> KKLNLKDKYQYLTRDMAWEPTYQDKKDIFPEEDFEGIKITDWSQWEDPFRLTMDAYWKYQAEKEKKLYAIFDAFAQNNGHQNISDARYVNALKLFISGISPLEHAAFQGYSKVGRQFSGAGARVACQMQAIDELRHSQTQQHAMSHYNKHFNGLHDGPHMHDRVWYLSVPKSFFDDARSAGPFEFLTAISFSFEYVLTNLLFVPFMSGAAYNGDMATVTFGFSAQSDEARHMTLGLEVIKFILEQHEDNVPIVQRWIDKWFWRGFRLLSLVSMMMDYMLPNKVMSWSEAWEVYYEQNGGALFKDLERYGIRPPKYQDVANDAKHHLSHQLWTTFYQYCQATNFHTW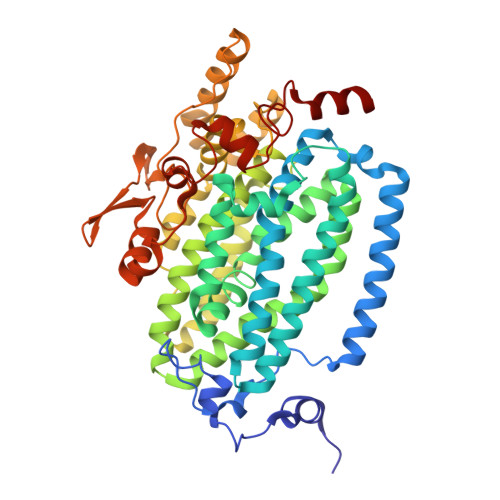IPEKEEMDWMSEKYPDTFDKYYRPRYEYLAKEAAAGRRFYNNTLPQLCQVCQIPTIFTEKDAPTMLSHRQIEHEGERYHFCSDGCCDIFKHEPEKYIQAWLPVHQIYQGNCEGGDLETVVQKYYHINIGEDNFDYVGSPDQKHWLSIK>DKIPDFVVPGKCASVDRNKLWAEQTPNRNSYAGVWYQFALTNNPYQLIEKCVR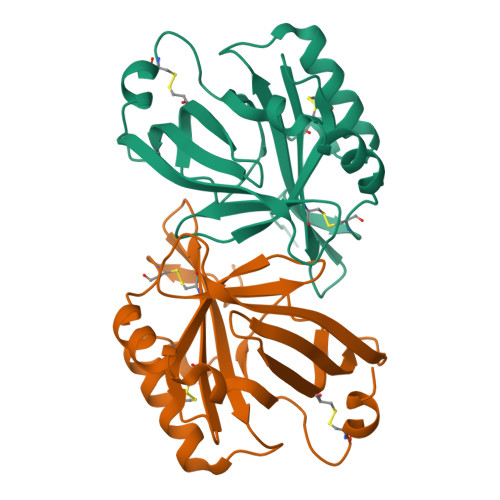NEYSFDGKQFVIESTGIAYDGNLLKRNGKLYPNPFGEPHLSIDYENSFAAPLVILETDYSNYACLYSCIDYNFGYHSDFSFIFSRSANLADQYVKKCEAAFKNINVDTTRFVKTVQGSSCPYDTQKTL[2x]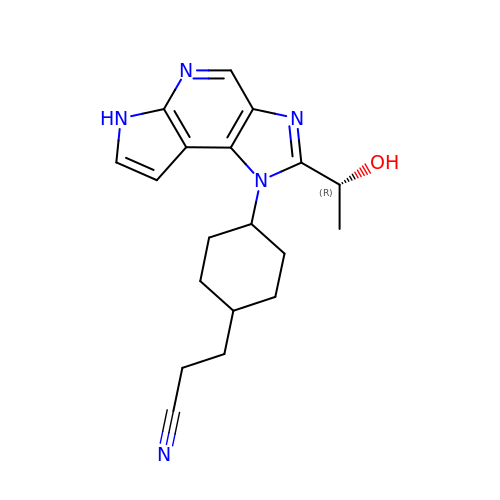3-(trans-4-{2-[(1R)-1-hydroxyethyl]imidazo[4,5-d]pyrrolo[2,3-b]pyridin-1(6H)-yl}cyclohexyl)propanenitrile | C19 H23 N5 O | LLRNGFSFYHDPKW-MGPQQGTHSA-N>PSLSKEAALVHEALVARGLETPLRPPVHEMDNETRKSLIAGHMTEIMQLLNLDLADDSLMETPHRIAKMYVDEIFSGLDYANFPKITLIENKMKVDEMVTVRDITLTSTCEHHFVTIDGKATVAYIPKDSVIGLSKINRIVQFFAQRPQVQERLTQQILIALQTLLGTNNVAVSIDAVHYSVKARGIRDATSATTTTSLGGLFKSSQNTRHEFLRAVRHHN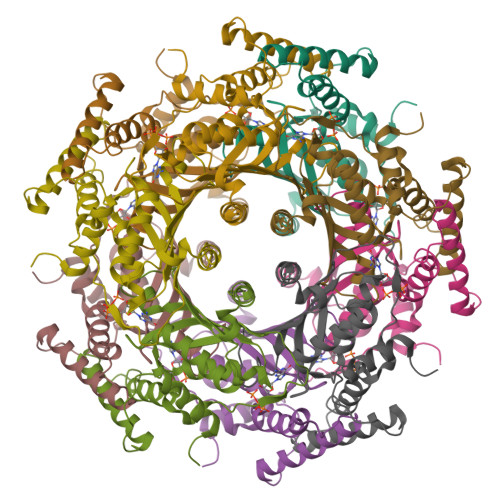[15x]6-[3-hydroxy-2-(hydroxymethyl)prop-1-en-1-yl]-5-methylpyrimidine-2,4(1H,3H)-dione 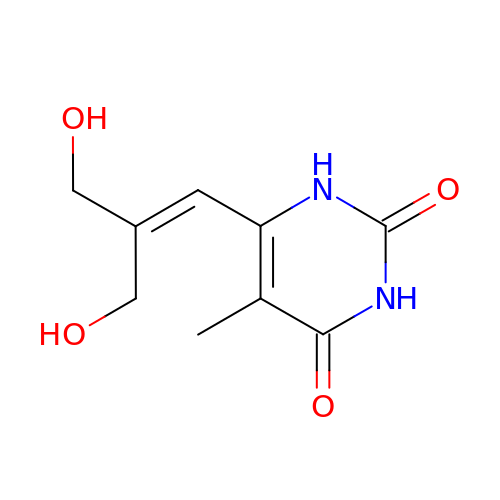| C9 H12 N2 O4 | IYYCMOUEXPXAQM-UHFFFAOYSA-N>[4x]MKHGILVAYKPKGPTSHDV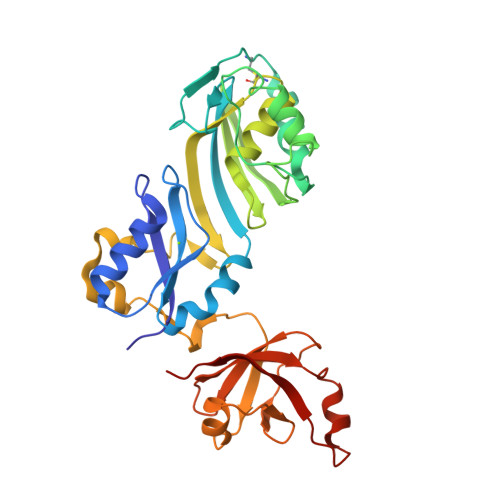VDEVRKKLKTRKVGHGGTLDPFACGVLIIGVNQGTRILEFYKDLKKVYWVKMRLGLITETFDITGEVVEERECNVTEEEIREAIFSFVGEYDQVPPAYSAKKYKGERLYKLAREGKIINLPPKRVKIFKIWDVNIEGRDVSFRVEVSPGTYIRSLCMDIGYKLGCGATAVELVRESVGPHTIEESLNVFEAAPEEIENRIIPLEKCLEWLPRVVVHQESTKMILNGSQIHLEMLKEWDGFKKGEVVRVFNEEGRLLALAEAERNSSFLETLRKHERQRRVLTLRKVFQTR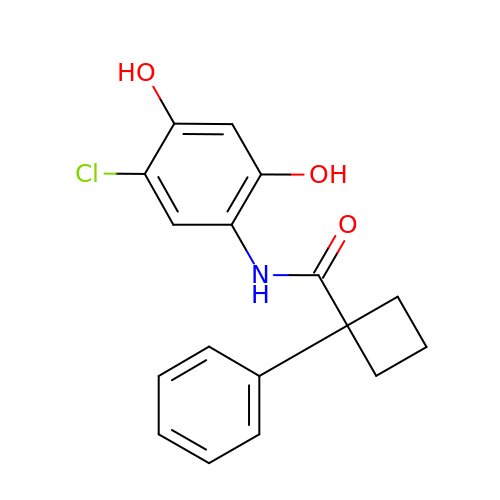N-(5-chloro-2,4-dihydroxyphenyl)-1-phenylcyclobutanecarboxamide | C17 H16 Cl N O3 | BOHOWRMNYYPMPP-UHFFFAOYSA-N> MSEASGTVRSFAHPGRGRNVARAVPKGRQVDPHAKVEIEELLGTRPRQRDLLIEHLHLIQDTYGQISADHLAALADEMSLAFAEVFETATFYAHFDVVKEGEADIPRLTIRVCDSITCAMFGADELLETLQRELASDAVRVVRAPCVGLCDHAPAVEVGHNFLHRADLASVRAAVEAEDTHAHIPTYVDYDAYRAGGGYATLERLRSGELPVDDVLKVLDDGGLRGLGGAGFPTGRKWRSVRGEPGPRLMAVNGDEGEPGTFKDQLYLNTDPHRFLEGMLIGAHVVEAADVYIYLRDEYPISREILAREIAKLPEGGTRIHLRRGAGAYICGEESSLIESLEGKRGLPRHKPPFPFQVGLFNRPTLINNIETLFWVRDLIERGAEWWKSHGRNGRVGLRSYSVSGRVKEPGVKLAPAGLTIQELIDEYCGGISDGHSFAA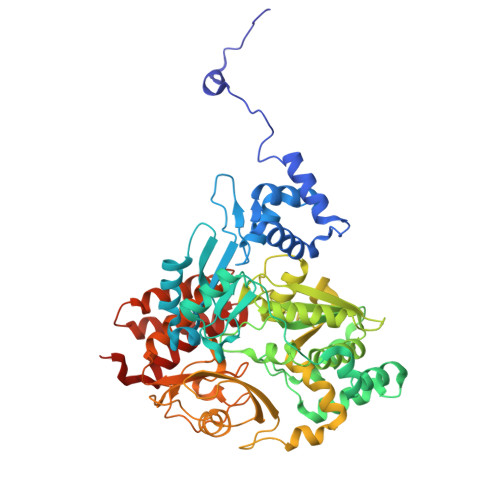YLPGGASGGILPASMNDIPLDFGTLEKYGCFIGSAAVVILSDQDDVRGAALNLMKFFEDESCGQCTPCRSGTQKARMLMENGVWDTDLLGELAQCMRDASICGLGQAASNPVSTVIKYFPDLFPEPRAVAAE> AKALIVYGSTTGNTEYTAETIARELADAGYEVDSRDAAS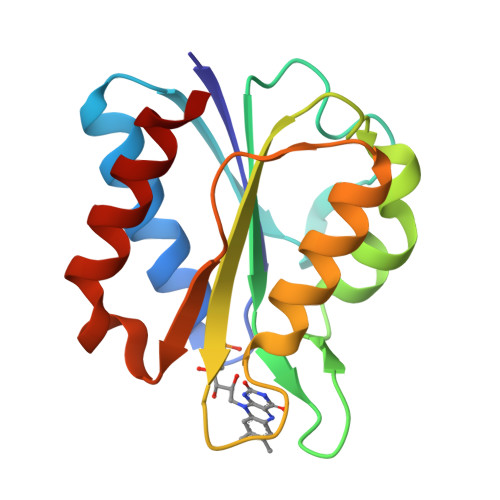VEAGGLFEGFDLVLLGCSTWGDDSIELQDDFIPLFDSLEETGAQGRKVACFGCGDSSYEYFCGAVDAIEEKLKNLGAEIVQDGLRIDGDPRAARDDIVGWAHDVRGAI> VDAELLADGKKVFAGNCAACHLGGNNSVLADKTLKKDAIE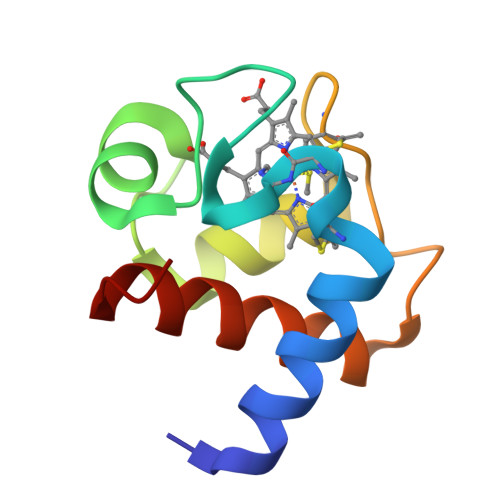KYLEGGLTLEAIKYQVNNGKGAMPAWADRLDEDDIEAVSNYVYDQAVNSKW> GSVADIQQLEEKV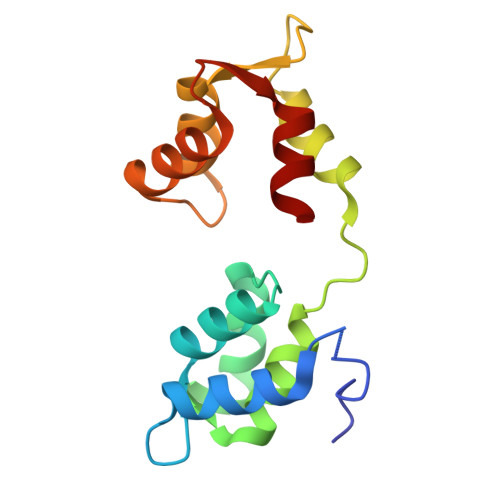DESDVRIYFNEKSSGGKISIDNASYNARKLGLAPSSIDEKKIKELYGDNLTYEQYLEYLSICVHDKDNVEELIKMFAHFDNNCTGYLTKSQMKNILTTWGDALTDQEAIDALNAFSSEDNIDYKLFCEDILQ> LKIQAYFNETADLPCQFANSQNQSLSELVVFW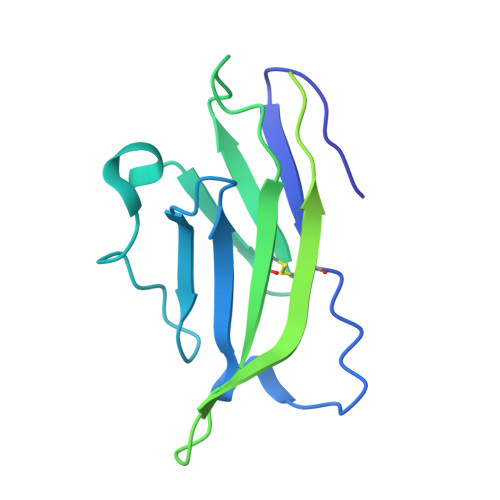QDQENLVLNEVYLGKEKFDSVHSKYMGRTSFDSDSWTLRLHNLQIKDKGLYQCIIHHKKPTGMIRIHQMNSELSVLANFSQPEIVPISNITENVYINLTCSSIHGYPEPKKMSVLLRTKNSTIEYDGVMQKSQDNVTELYDVSISLSVSFPDVTSNMTIFCILETDKTRLLSSPFSIELED(3S)-N-[3-(trifluoromethoxy)benzyl]-1-{2-[(3,4,5-trimethoxyphenyl)amino]pyrimidin-4-yl}piperidine-3-carboxamide 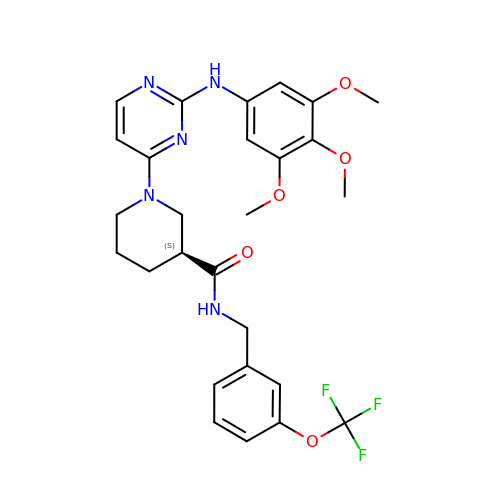| C27 H30 F3 N5 O5 | LDRVTAIULYJYRP-SFHVURJKSA-N5-CHLORO-1H-INDOLE-2-CARBOXYLIC 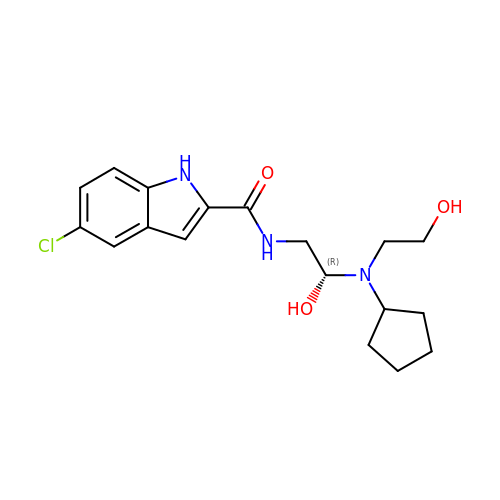ACID{[CYCLOPENTYL-(2-HYDROXY-ETHYL)-CARBAMOYL]-METHYL}-AMIDE | C18 H24 Cl N3 O3 | VXABTOCIIZSEPD-QGZVFWFLSA-N>MEEPFEAYRSREVAMKLVEKIREEAKTLDGEIRIMHVCGTHEDTVTRHGIRSLLPENVKVVSGPGCPVCITPVEDIVAMQLIMRKAREEGEEIILTTFGDMYKIPTPMGSFADLKSEGFDVRIVYGIFDTYRIAKENPDKTVVHFSPGFETTTAPAAGMLNVAAQEELENFKIYSVHRLTPPAVEVLLKQGTVFQGLIAPGHVSTIIGVKGWEYLTEKYGIPQVVAGFEPNDVLMAILMLIRMYKEGEARIINEYERAVKYEGNVVAQKMIDKFFEVVDAKWRALGVFPKSGLELRKEWKDFEIRSFYKVEVPKNLPDLEKGCRCGAVLRGLALPTDCPLFGKTCTP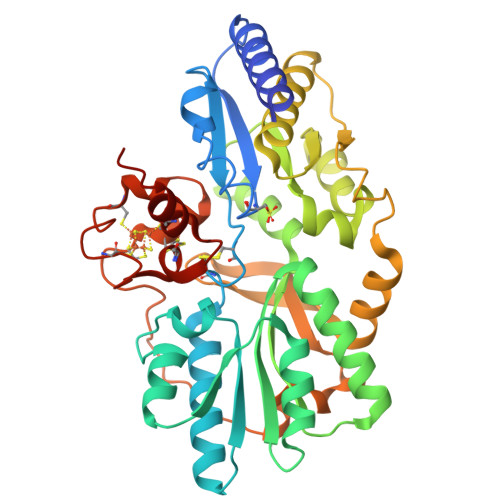RHPVGPCMVSYEGTCQIFYKYGVLF[2x]>[2x]KDCFKEKNEKEMEEEAEMKAVATSPSGRFLKFDIELGRGAFKTVYKGLDTETWVEVAWCELQDRKLTKAEQQRFKEEAEMLKGLQHPNIVRFYDSWESILKGKKCIVLVTELM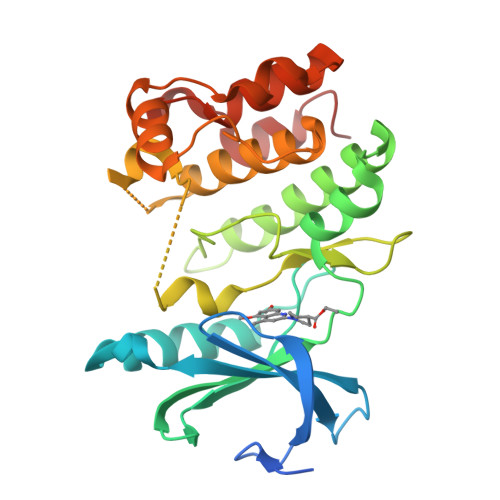TSGTLKTYLKRFKVMKPKVLRSWCRQILKGLQFLHTRTPPIIHRDLKCDNIFITGPTGSVKIGDLGLATLMRTSFAKAVIGTPEFMAPEMYEEHYDESVDVYAFGMCMLEMATSEYPYSECQNAAQIYRKVTSGIKPASFNKVTDPEVKEIIEGCIRQNKSERLSIRDLLNHAFFAEDT6-fluoro-1H-benzimidazol-2-amine | C7 H6 F N3 | 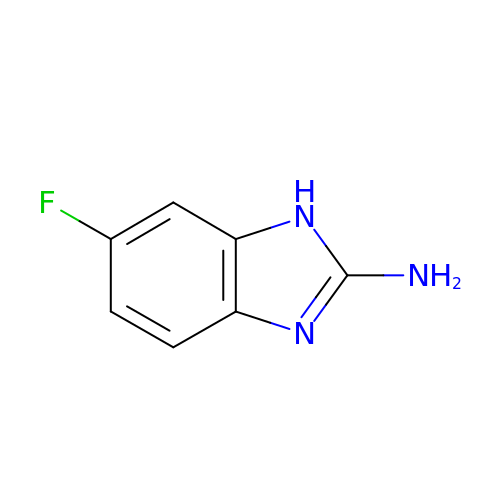MKYGXXIXMHTQFA-UHFFFAOYSA-N> MNIDGLDALLNQFHDMKTNIDDDVDDILQENAKEYVVRAKLKARE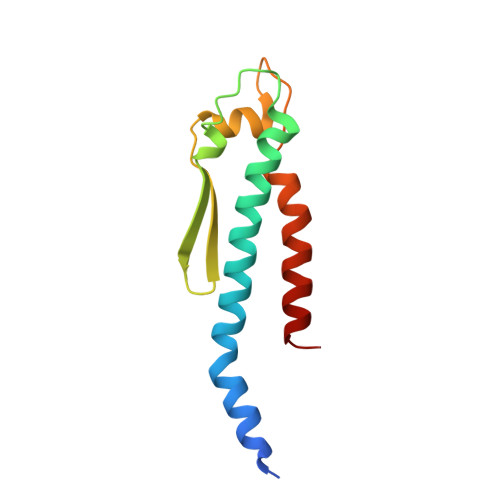VMNKGYWTGNLSRNIRYKKTGDLQYTITSHAAYSGFLEFGTRYMEAEPFMWPVYEVIRKSTVEELKALFE PHOSPHORIC ACID 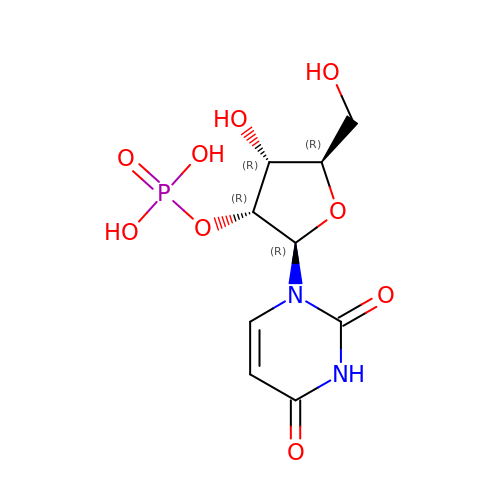MONO-[2-(2,4-DIOXO-3,4-DIHYDRO-2H-PYRIMIDIN-1-YL)-4-HYDROXY-5-HYDROXYMETHYL-TETRAHYDRO-FURAN-3-YL] ESTER | C9 H13 N2 O9 P | HQIDPEYTETUCNF-XVFCMESISA-N> GIDPNYRTNRQVVGEHSGHKVYGPVEPPKVLGIHGTIVGVDFDLCIADGSCINACPVNVFQWYDTPGHPASEKKAD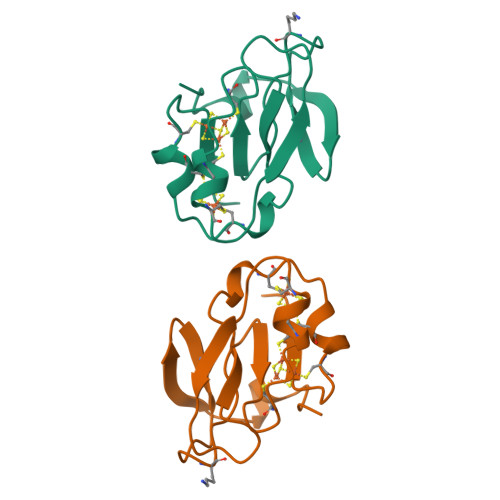PVNEQACIFCMACVNVCPVAAIDVKPP>[3x]QTE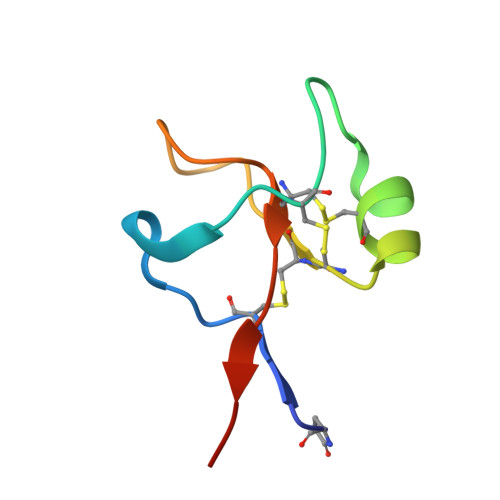TCTVAPRERQNCGFPGVTPSQCANKGCCFDDTVRGVPWCFYPNTILEK>XGELAQSLKELAKSLKELAWSLKELAQSLKGX[3x]

CCs are quaternary structures comprising two or more α-helices supercoiled around each other with cyclic (Cn) or dihedral (Dn) symmetry. Here, we describe variants with all combinations of the aliphatic residues, Ile, Leu and Val, at a and d to give four classes of peptide: the ββ class, with a and d = Ile or Val; Lβ, a = Leu and d = Ile or Val; βL, a = Ile or Val and d = Leu; and LL, a = d = Leu. Peptides are named systematically appending the one-letter code for the amino acids at the a and d sites to “CC-Type2-“; e.g., CC-Hept becomes CC-Type2-LI. In summary, solution-phase data and X-ray crystal structures demonstrate conclusively that different classes of Type-2 coiled-coil (CC) peptides—i.e., based on abcdefg repeats with predominantly hydrophobic residues at a, d, e and g—adopt a range of distinct states.

Completing these variations, CC-Type2-LL-Sg (LL-class) is another structure with reduced C2 symmetry, comprising two 3-helix layers. The two collapsed structures were more complicated. Nonetheless, both had extensive KIH interfaces linking all helices and, as such, are CC-based structures. And LL sequences form collapsed structures. However, the cognate structure for each sequence did not always have the lowest score, as apparent from the off-diagonal white and blue points. This occurs for all of the LL-based sequences and those βL sequences observed to form collapsed structures. For these, we propose that the collapsed states are adopted as they lead to more hydrophobic burial and contacts. Inspection of the models for these alternative states exposed steric clashes associated with the β-branched residues; e.g., threading of the CC-Type2-II sequence onto the CC-Type2-LL-Sg structure resulted in irreconcilable clashes between Cδ and Cγ1 atoms of Ile residues at a and d’ sites of neighbouring helices.>[6x]TSRNYLLLTPGPLTTSRTVKEAMLFDSCTWDDDYNIGVVEQIRQQLTALATASEGYTSVLLQGSGSYAVEAVLGSALGPQDKVLIVSNGAYGARMVEMAGLMGIAHHAYDCGEVARPDVQAIDAILNADPTISHIAMVHSETTTGMLNPIDEVGALAHRYGKTYIVDAMSSFGGIPMDIAALHIDYLISSANKCIQGVPGFAFVIAREQKLAACKGHSRSLS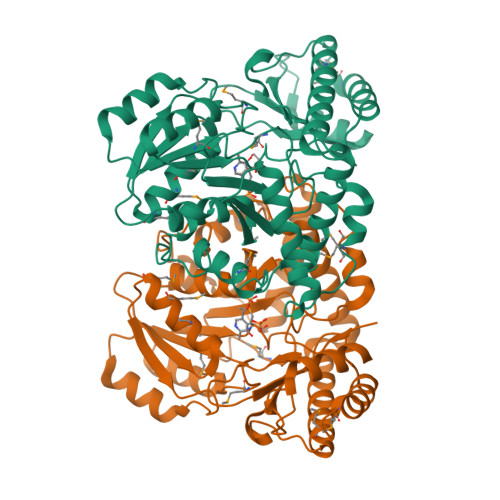LDLYAQWRCMEDNHGKWRFTSPTHTVLAFAQALKELAKEGGVAARHQRYQQNQRSLVAGMRALGFNTLLDDELHSPIITAFYSPEDPQYRFSEFYRRLKEQGFVIYPGKVSQSDCFRIGNIGEVYAADITALLTAIRTAMYWTK>TTQPALLRLSDHLLANYKKGVRPVRDWRKPTTVSIDVIMYAILNVDEKNQVLTTYIWYRQYWTDEFLQWTPEDFDNVTKLSIPTDSIWVPDILINEFVDVGKSPNIPYVYVHHRGEVQNYKPLQLVTACSLDIYNFPFDVQNCSLTFTSWLHTIQDINITLWRSPEEVRSDKSIFINQGEWELLEVFPQFKEFSIDISNSYAEMKFYVIIRRRPLFYAVSLLLPSIFLMVVDIVGFCLPPDSGERVSFKITLLLGYSVFLIIVSDTLPATAIGTPLIGVYFVVCMALLVISLAETIFIVRLVHKQDLQRPVPDWLRHLVLDRIAWILCLGEQPMAHRPPATFQANKTDDCSAMGNHCSHVGGPQDLEKTPRGRGSPLPPPREASLAVRGLLQELSSIRHFLEKRDEMREVARDWLRVGYVLDRLLFRIYLLAVLAYSITLVTLWSIWHYS[5x]

Serotonin binds to serotonin receptors (5-HT3Rs), a pentameric ligand-gated ion channel (pLGIC), on the vagal afferent nerve in the gut and on the chemoreceptor trigger zone in the brainstem leading to severe nausea and vomiting in patients receiving cancer treatments. Setrons, competitive antagonists of 5-HT3R, are effective in the prevention of chemotherapy-induced nausea and vomiting (CINV), radiation therapy- induced nausea and vomiting (RINV), and postoperative nausea and vomiting (PONV). In the present study, we have solved cryo-EM structures of the full-length 5-HT3AR in complex with palonosetron, ondansetron, and alosetron at the resolution range of 2.9 Å to 3.3 Å. Overall, setrons stabilize 5-HT3AR conformational states that are non-conductive, but appear to lie between the apo and serotonin-bound states.

For example, the FDA approved treatment of diarrhea-predominant IBS with alosetron led to severe ischemic colitis in many patients. Iterative classifications and C5 symmetry-imposed refinement produced a final three-dimensional reconstruction at a nominal resolution of 3.3 Å for 5-HT3AR-Palono (with 91,163 particles), 3.0 Å for 5-HT3AR-Ondan (67,333 particles), and 2.9 Å for 5-HT3AR-Alo (42,065 particles). The aromatic end of the molecule is an indazole in granisetron, isoquinoline in palonosetron, carbazole in ondansetron, and pyridoindole in alosetron. In particular, the carbonyl oxygen of Trp156 is close to the amine group of setron, and in the 5-HT3AR-Alo, it forms a hydrogen bond with the amine group in the diazole ring. In 5-HT3AR-Alo, one of the secondary amine nitrogen on the diazole ring forms a water-mediated hydrogen-bond interaction with the carbonyl oxygen of Trp156. The backbone oxygen of Tyr64 interacts with the carbonyl group of the ligand’s pyridoindole ring through a water molecule. Interestingly, water-mediated interactions with Glu209 are absent in the alosetron fingerprint when compared to the ondansetron, granisetron, and serotonin fingerprints. In comparison to the 5-HT3AR-Apo structure, Loop C adopts varying degrees of an inward conformation, and in the 5-HT3AR-Alo structure the orientation is similar to 5-HT3AR-serotonin (Basak et al., 2019). Comparing these two parameters across the different systems suggest that Loop C is stable in its initial cryo-EM conformation in the case of 5-HT3AR-Alo and 5-HT3AR-Serotonin simulations where it predominantly adopts a ‘closed’ conformation. We find that the 5-HT3AR-Alo and 5-HT3AR-Serotonin MD simulations maintained an interaction between Arg65 and Asp202 more often than in any other setron-bound structure, and that most setron-bound simulations did not appreciably form this stabilizing interaction.>ETGQKLDDVDPLVATNFGKIRGIKKELNNEILGPVIQFLGVPYAAPPTGERRFQPPEPPSPWSDIRNATQFAPVCPQNIIDGRLPEVMLPVWFTNNLDVVSSYVQDQSEDCLYLN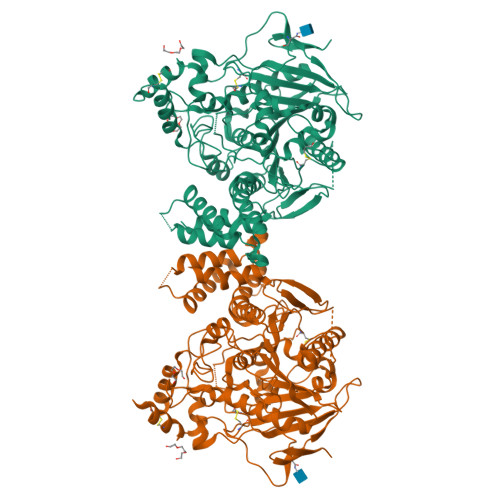IYVPTEDDIRDSGGPKPVMVYIHGGSYMEGTGNLYDGSVLASYGNVIVITVNYRLGVLGFLSTGDQAAKGNYGLLDLIQALRWTSENIGFFGGDPLRITVFGSGAGGSCVNLLTLSHYSEGNRWSNSTKGLFQRAIAQSGTALSSWAVSFQPAKYARMLATKVGCNVSDTVELVECLQKKPYKELVDQDIQPARYHIAFGPVIDGDVIPDDPQILMEQGEFLNYDIMLGVNQGEGLKFVENIVDSDDGISASDFDFAVSNFVDNLYGYPEGKDVLRETIKFMYTDWADRHNPETRRKTLLALFTDHQWVAPAVATADLHSNFGSPTYFYAFYHHCQTDQVPAWADAAHGDEVPYVLGIPMIGPTELFPCNFSKNDVMLSAVVMTYWTNFAKTGDPNQPVPQDTKFIHTKPNRFEEVAWTRYSQKDQLYLHIGLKPRVKEHYRANKVNLWLELVPHLHNLNDRTKHHHHHH[2x]>[6x]MFVLSGGRWEKTDLTYRILR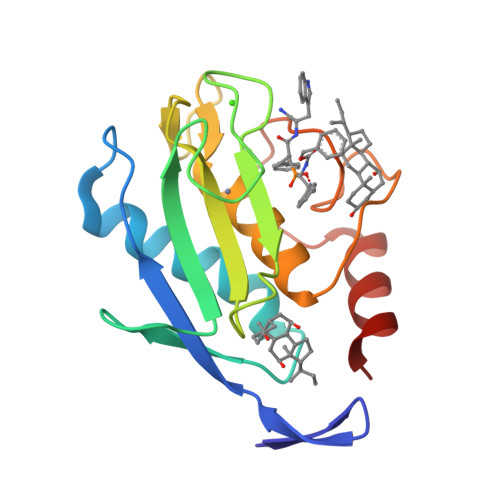FPWQLVREQVRQTVAEALQVWSEVTPLTFTEVHEGRADIMIDFARYWHGDNLPFDGPGGILAHAFFPKTHREGDVHFDYDETWTIGDNQGTDLLQVAAHEFGHVLGLQHTTAAKALMSPFYTFRYPLSLSPDDRRGIQHLYGRPQ> MSGMLDELFSLLNKMFELSDKYRELRKELRKAIESGAPEEELRELLEKMLEIAKKLLELTKELKKLVEDVLKNNPDPVERAKAVLLYAVGVHILYSESSELEVIAERLG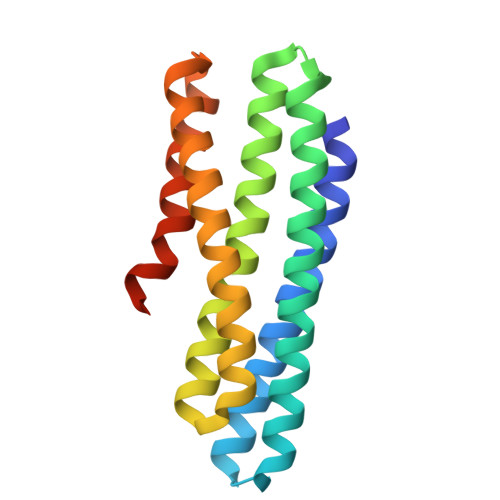FKDIAEKAKEIADKARELKEEVKRKLREIREEVPDPEIRKAAEEAIEMLESNDKRLKEFRKLHSQ> AQYYPGTTKVAQNRRNFCNPEYELEKLREISDEDVVKILGHRAPGEEYPSVHPPLEEMDEPEDAIREMVEPIDGAKAGDRVRYIQFTDSMYFAPAQPYVRSRAYLCRYRGADAGTLSGRQIIETRERDLEKISKELLETEFFDPARSGVRGKSVHGHSLRLDEDGMMFDMLRRQIYNKDTGRV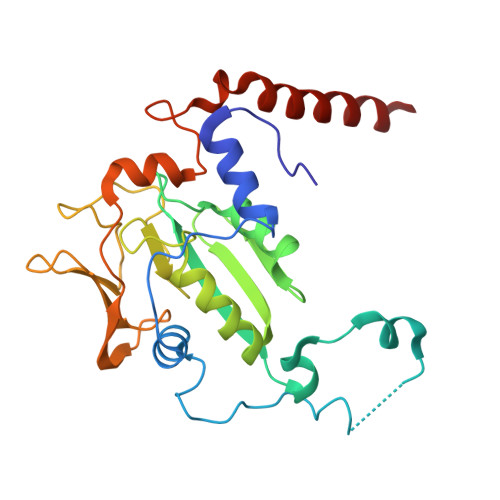EMVKNQIGDELDEPVDLGEPLDEETLMEKTTIYRVDGEAYRDDVEAVEIMQRIHVLRSQGGFN>[3x]MLSNELRQTLQKGLHDVNSDWTVPAAIINDPEVHDVERERIFGHAWVFLAHESEIPERGDYVVRYISEDQFIVCRDEGGEIRGHLNACRHRGMQVCRAEMGNTSHFRCPYHGWTYSNTGSLVGVPAGKDAYGNQLKKSDWNLRPMPNLASYKGLIFGSLDPHADSLEDYLGDLKFYLDIVLDRSDAGLQVVGAPQRWVIDANWKLGADNFVGDAYHTMMTHRSMVELGLAPPDPQFALYGEHIHTGHGHGLGIIGPPPGMPLPEFMGLPENIVEELERRLTPEQVEIFRPTAFIHGTVFPNLSIGNFLMGKDHLSAPTAFLTLRLWHPLGPDKMEVMSFFLVEKDAPDWFKDESYKSYLRTFGISGGFEQDDAENWRSITRVMGGQFAKTGELNYQMGRGVLEPDPNWTGPGEAYPLDY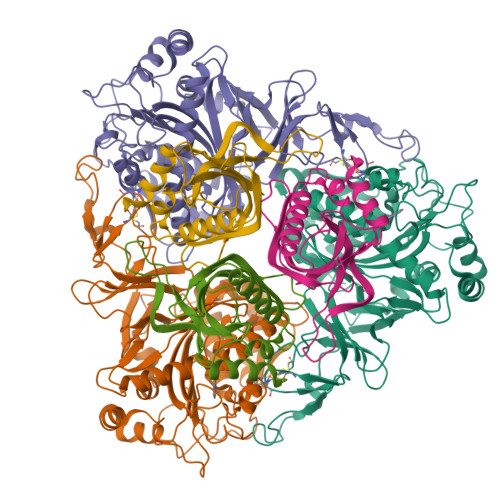AEANQRNFLEYWMQLMLAESPLRDGNSNGSGTADASTPAAAKSKSPAKAEA;>MNTQTRVSDTTVREITEWLYMEAELLDAGKYREWLALVTEDLSYVVPIRVTREREAVTDVVEGMTHMDDDADSMEMRVLRLETEYAWAEDPPSRSRHFVTNVRVATGDSEDEFKVTSNLLLYRTRGDVATYDVLSGERTDVLRRAGDSFLMAKRVVLLDQTTIMTHNLALIM[3x]> MPLYVIDKPITLHILTQLRDKYTDQINFRKNLVRLGRILGYEISNTLDYEIVEVETPLGVKT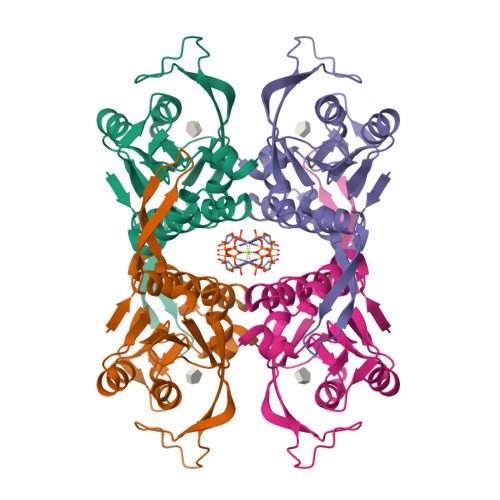KGVDITDLNNIVIINILRAAVPLVEGLLKAFPKARQGVIGASRVEVDGKEVPKDMDVYIYYKKIPDIRAKVDNVIIADPMIATASTMLKVLEEVVKANPKRIYIVSIISSEYGVNKILSKYPFIYLFTVAIDPELNNKGYILPGLGDAGDRAFG> MISATYRLQLNKNFNFGDVIDNLWYFKDLGVSHLYLSPVLMASPGSNHGYDVIDHSRINDELGGEKEYRRLIETAHTIGLGIIQDIVPNHMAVNSLNWRLMDVLKMGKKSKYYTYFDFFPEDDKIRLPILGEDLDTVISKGLLKIVKDGDEYFLEYFKWKLPLTEVGNDIYDTLQKQNYTLMSWKNPPSYRRFFDVNTLIGVNVEKDHVFQESHSKILDLDVDGYRIDHIDGLYDPEKYINDLRSIIKNKIIIVEKILGFQEELKLNSDGTTGYDFLNYSNLLFNFNQEIMDSIYENFTAEKISISESIKKIKAQIIDELFSYEVKRLASQLGISYDILRDYLSCIDVYRTYANQIVKECDKTNEIEEATKRNPEAYTKLQQYMPAVYAKAYEDTFLFRYNRLISINEVGSDLRYYKISPDQFHVFNQKRRGKITLNATSTHDTKFSEDVRMKISVLSEFPEEWKNKVEEWHSIINPKVSRNDEYRYYQ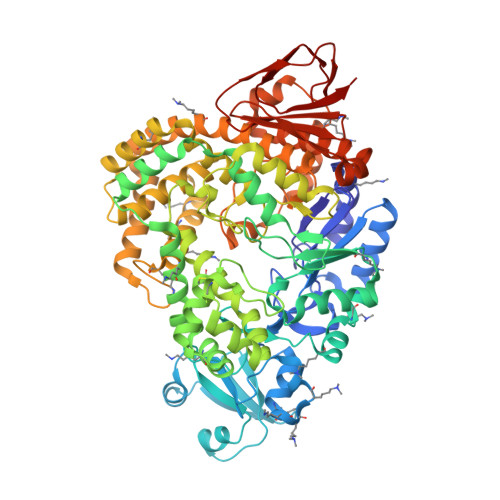VLVGSFYEGFSNDFKERIKQHMIKSVREAKINTSWRNQNKEYENRVMELVEETFTNKDFIKSFMKFESKIRRIGMIKSLSLVALKIMSAGIPDFYQGTEIWRYLLTDPDNRVPVDFKKLHEILEKSKKFEKNMLESMDDGRIKMYLTYKLLSLRKQLAEDFLKGEYKGLDLEEGLCGFIRFNKILVIIKTKGSVNYKLKLEEGAIYTDVLTGEEIKKEVQINELPRILVRM> MSFDRPEIYSAPVLQGESPNDDDNTEIIKSFKNFILEFRLDSQFIYRDQLRNNILVKNYSLTVNMEHLIGYNEDIYKKLSDEPSDIIPLFETAITQVAKRISILSRAQSANNNDKDPENTSMDTDSLLLNSLPTFQLILNSNANQIPLRDLDSEHVSKIVRLSGIIISTSVLSSRATYLSIMCRNCRHTTSITINNFNSITGNTVSLPRSCLSTIESESSMANESNIGDESTKKNCGPDPYIIIHESSKFIDQQFLKLQEIPELVPVGEMPRNLTMTCDRYLTNKVIPGTRVTIVGIYSIYNSKNGAGSGRSGGGNGGSGVAIRTPYIKILGIQSDVETSSIWNSVTMFTEEEEEEFLQLSRNPKLYEILTNSIAPSIFGNEDIKKAIVCLLMGGSKKILPDGMRLRGDINVLLLGDPGTAKSQLLKFVEKVSPIAVYTSGKGSSAAGLTASVQRDPMTREFYLEGGAMVLADGGVVCIDEFDKMRDEDRVAIHEAMEQQTISIAKAGITTVLNSRTSVLAAANPIYGRYDDLKSPGDNIDFQTTILSRF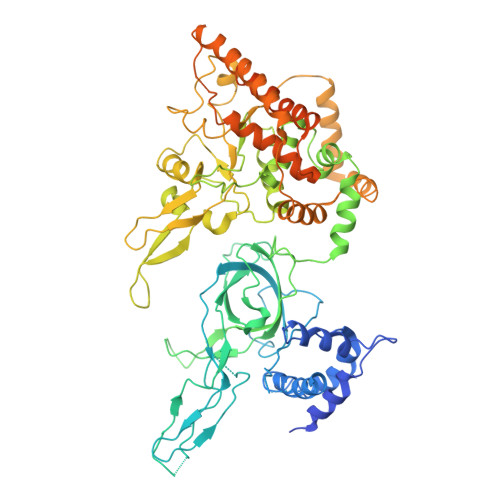DMIFIVKDDHNEERDISIANHVINIHTGNANAMQNQQEENGSEISIEKMKRYITYCRLKCAPRLSPQAAEKLSSNFVTIRKQLLINELESTERSSIPITIRQLEAIIRITESLAKLELSPIAQERHVDEAIRLFQASTMDAASQDPIGGLNQASGTSLSEIRRFEQELKRRLPIGWSTSYQTLRREFVDTHRFSQLALDKALYALEKHETIQLRHQGQNIYRSGV> NSLDRAQAAKNKGNKYFKAGKYEQAIQCYTEAISLCPTEKNVDLSTFYQNRAAAFEQLQKWKEVAQDCTKAVELNPKYVKALFRRAKAHEKLDNKKECLEDVTAVCILEGFQNQQSMLLADKVLKLLGKEKAKEKYKNREPLMPSPQFIKSYFSSFTDDIISQPMLKGEKSDEDKDKEGEALEVKENSGYLKAKQYMEEENYDKIISECSKEIDAEGKYMAEALLLRATFYLLIGNANAAKPDLDKVISLKEANVKLRANALIKRGSMYMQQQQPLLSTQDFNMAADIDPQNADVYHHRGQLKILLDQVEEAVADFDECIRLRPESALAQAQKCFA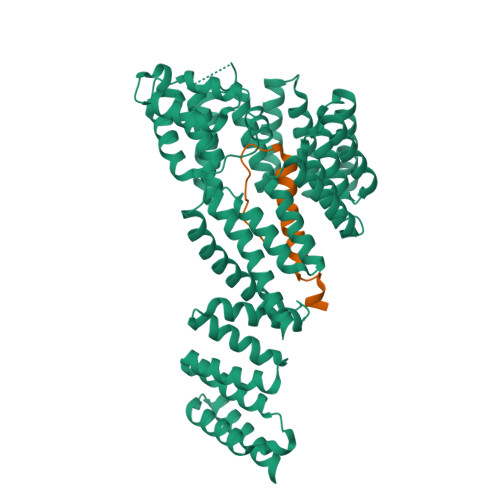LYRQAYTGNNSSQIQAAMKGFEEVIKKFPRCAEGYALYAQALTDQQQFGKADEMYDKCIDLEPDNATTYVHKGLLQLQWKQDLDRGLELISKAIEIDNKCDFAYETMGTIEVQRGNMEKAIDMFNKAINLAKSEMEMAHLYSLCDAAHAQTEVAKKYGLKPPTL;> MDPKISEMHPALRLVDPQIQLAVTRMENAVGRDQNNVGPKVYPIILRLGSPLSLNMARKTLNSLEDKAFQLTPIAVQMTKLATTEELPDEFVVVTVK> GSLVLYGAPYERAVEVLEETLRETGARYALLIDRKGFVLAHKEALWAPKPPPLDTLATLVASNAAATQALAKLLGEARFQEEVHQGERMGLYVDEAGEHALLVLVFDETAPLGKVKLHGKAAAAALARIAE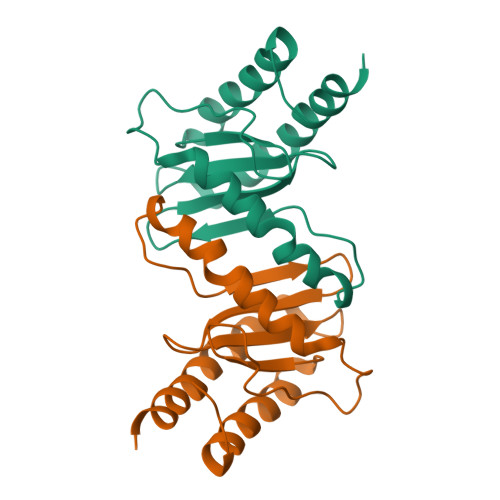EALAN>[6x]MAAIQGIEGVISQLQATAMAARGQDTHSQSTVSFAGQLHAALDRISDRQAAARVQAEKFTLGEP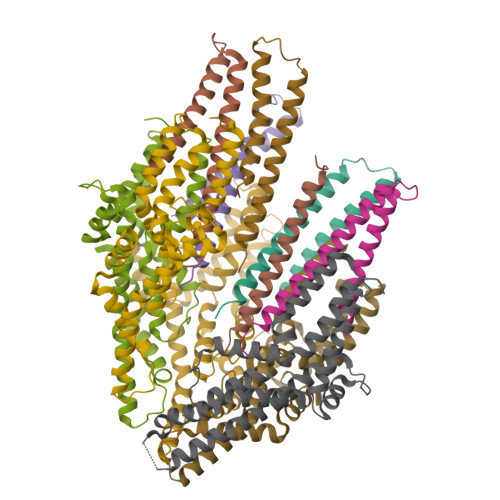GIALNDVMADMQKASVSMQMGIQVRNKLVAAYQEVMSMQV;>MRRLLFLSLAGLWLFSPAAAAQLPGLISQPLAGGGQSWSLSVQTLVFITSLTFLPAILLMMTSFTRIIIVFGLLRNALGTPSAPPNQVLLGLALFLTFFIMSPVIDKIYVDAYQPFSEQKISMQEALDKGAQPLRAFMLRQTREADLALFARLANSGPLQGPEAVPMRILLPAYVTSELKTAFQIGFTIFIPFLIIDLVIASVLMALGMMMVPPATIALPFKLMLFVLVDGWQLLMGSLAQSFYS[5x]> SNAMFAPQGLAQFIKVNVTLENGEPVFIYTDANGQVCQGDITVTQAGTITYLLNDQTLKGLKFV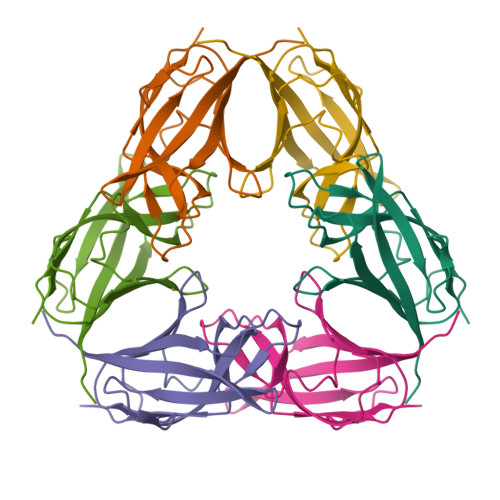GVGFVTPFDGIIDAVTISSDGMLVQLVDLDKTPGTTKFQFVLSNTANTLLVLSPDAQIINRPQN>[2x]MDVDLPPPGPLTSGGLRVTALGGINEIGRNMTVFEHLGRLLIIDCGVLFPGHDEPGVDLILPDMRHVEDRLDDIEALVLTHGHEDHIGAIPFLLKLRPDIPVVGSKFTLALVAEKCREYRITPVFVEVREGQSTRHGVFECEYFAVNHSTPDALAIAVYTGAGTILHTGDIKFDQLPPDGRPTDLPGMSRLGDTGVDLLLCDSTNAEIPGVGPSESEVGPTLHRLIRGADGRVIVACFASNVDRVQQIIDAAVALGRRVSFVGRSMVRNMRVARQLGFLRVADSDLIDIAAAETMAPDQVVLITTGTQGEPMSALSRMSRGEHRSITLTAGDLIVLSSSLIPGNEEAVFGVIDA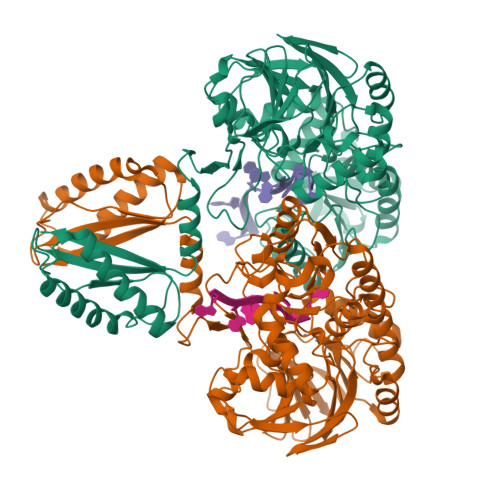LSKIGARVVTNAQARVHVSGHAYAGELLFLYNGVRPRNVMPVHGTWRMLRANAKLAASTGVPQESILLAENGVSVDLVAGKASISGAVPVGKMFVDGLIAGDVGDITLGERLILSSGFVAVTVVVRRGTGQPLAAPHLHSRGFSEDPKALEPAVRKVEAELESLVAANVTDPIRIAQGVRRTVGKWVGETYRRQPMIVPTVIEV SisCsx1, as other members of the Csm6/Csx1 family, is composed of an N-terminal CRISPR-Cas-associated Rossmann Fold (CARF) domain connected to an α-helical higher eukaryotes and prokaryotes nucleotide-binding (HEPN) domain by a helix-turn-helix (HTH) domain. The SisCsx1 monomers are curled around the two-fold axis to form a dimer, and three of these dimers oligomerize through their HEPN domains into an equilateral trimer, thus assembling into a hexamer. Each dimer contains a cOA4 binding site at the vertex of the triangular assembly, and a catalytic pocket located 70 Å away inside the triangular oligomer along the two-fold dimer axis. We show that cOA4 binding activates a cooperative sequential catalytic response in a hexameric SisCsx1 complex and that the RNase activity is switched-off by Ring nucleases, which cleave cOA423.

A cryoEM map of the complex at medium resolution was used as a model to solve the phase problem by molecular replacement in an apo SisCsx1 crystal belonging to the P21 space group. The Cα backbone built in this map was later combined with an iodine derivative of a better diffracting crystal of SisCsx1 in the space group I212121 to determine the structure of the apo SisCsx1 to 2.9 Å. The cOA4 binding cleft is formed by the loops connecting several secondary structure elements of the CARF domains, including residues in loops spanning residues 6–18, 28–30, 47–54, 92–100, 153–158 and 178–188. The conformational changes upon cOA4 binding induce a reshaping of the loops, so that the oval cleft observed in the apo structure shifts to form a cruciform pocket, in which the cOA4 is bound. The active center cleft comprises R354, D372, R389, R399, N400, M403, H404, T409, and D410 residues. The SisCsx1 dimeric arrangement results in a symmetric placement of these amino acids, creating a diagonal electropositive stripe flanked by two electronegative regions on each side.

>[3x]MKCLFYIAGDVSNYSIVNYELNGQTQNTFFAAHALYNLFKPDKVIALIPDSLVKDNVSDEECYKNLVINRAKELNFAGMEEFMNKVEIRKIPNVGIASAIQCENGAPKKEKNKEGREVLKRLPYNEKRSPIFIFNAIYAIFKDEACDEYLVDLTHGTNVLVSIGMNVGALFNAKFYSAPVMGMPGKDSIVNIVELTDVVQATNDSLMIRSSIENLDERYFKDYSAKLSRLNPTIFEEEEKKVLTRVKGTDVNVVINFLWNIRNGFTVNAVKSMNELKNIINQLEEDLEKLKSFYKNWEEHKNFQGETLLVLSDLDSTLKVKDLLIEGNDLEKLNYLLDLYIKASIYDKALSLARELPVAICLNKVGGGMFDDKNEKYKHCNEIVTSYLRLRYSGLMEFRNTLMHGGLSTDMKPNVDKDGNITPGKIVTKNKIEDFVKRELRNYFDKIVNFLSSA> PIMLEDY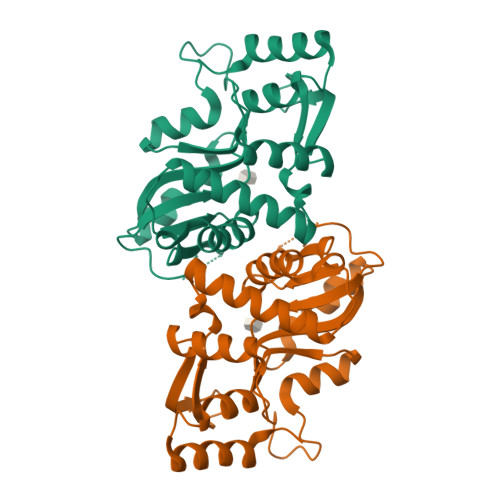QKNFLELAIECQALRFGSFKLKSGRESPYFFNLGLFNTGKLLSNLATAYAIAIIQSDLKFDVIFGPAYKGIPLAAIVCVKLAEIGGSKFQNIQYAFNRKEAKDHGEGGIIVGSALENKRILIIDDVMTAGTAINEAFEIISNAKGQVVGSIIALDRQEVVSTDDKEGLSATQTVSKKYGIPVLSIVSLIHIITYLEGRITAEEKSKIEQYLQTYGASAENLYFQ> MEDPVTGPEEVSGQEQGSLTVQCRYTSGWKDYKKYWCQGVPQRSCKTLVETDASEQLVKKNRVSIRDNQRDFIFTVTMEDLR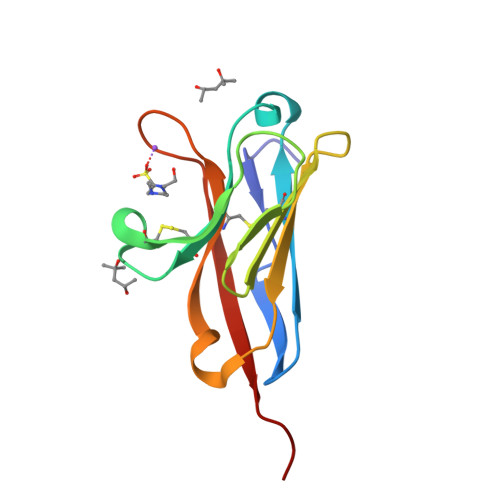MSDAGIYWCGITKGGLDPMFKVTVNIGPVPT>[2x]SVVVISQALPVPTRIPGVADLVGFGNGGVYIIRNSLLIQVVKVINNFGYDAGGWRVEKHVRLLADTTGDNQPDVVGFGENGVWISTNNGNNTFVDPPKMVLANFAYAAGGWRVEKHIRFMADLRKTGRADIVGFGDGGIYISRNNGGGQFAPAQL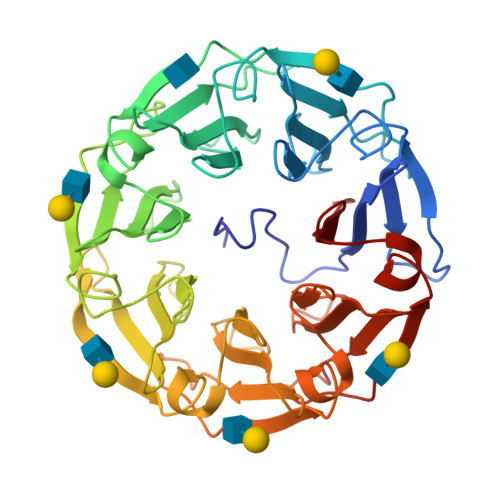ALNNFGYAQGWRLDRHLRFLADVTGDGLLDVVGFGENQVYIARNSGNGTFQPAQAVVNNFCIGAGGWTISAHPRVVADLTGDRKADILGFGVAGVYTSLNNGNGTFGAVNLVLKDFGVNSGWRVEKHVRCVSSLTNKKVGDIIGFGDAGVYVALNNGNGTFGPVKRVIDNFGYNQGWRVDKHPRFVVDLTGDGCADIVGFGENSVWACMNKGDGTFGPIMQLIDDMTVSKGWTLQKTVRYAANLYL> MGTVSSRRSWWPLPLLLLLLLLLGPAGARAQEDEDGDYEELVLALRSEEDGLAEAPEHGTTATFHRCAKDPWRLPGTYV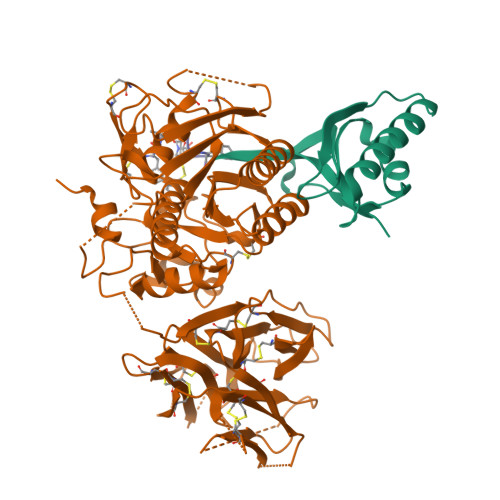VVLKEETHLSQSERTARRLQAQAARRGYLTKILHVFHGLLPGFLVKMSGDLLELALKLPHVDYIEEDSSVFAQ;> SIPWNLERITPPRYRADEYQPPDGGSLVEVYLLDTSIQSDHREIEGRVMVTDFENVPEEDGTRFHRQASKCDSHGTHLAGVVSGRDAGVAKGASMRSLRVLNCQGKGTVSGTLIGLEFIRKSQLVQPVGPLVVLLPLAGGYSRVLNAACQRLARAGVVLVTAAGNFRDDACLYSPASAPEVITVGATNAQDQPVTLGTLGTNFGRCVDLFAPGEDIIGASSDCSTCFVSQSGTSQAAAHVAGIAAMMLSAEPELTLAELRQRLIHFSAKDVINEAWFPEDQRVLTPNLVAALPPSTHGAGWQLFCRTVWSAHSGPTRMATAIARCAPDEELLSCSSFSRSGKRRGERMEAQGGKLVCRAHNAFGGEGVYAIARCCLLPQANCSVHTAPPAEASMGTRVHCHQQGHVLTGCSSHWEVEDLGTHKPPVLRPRGQPNQCVGHREASIHASCCHAPGLECKVKEHGIPAPQEQVTVACEEGWTLTGCSALPGTSHVLGAYAVDNTCVVRSRDVSTTGSTSEEAVTAVAICCRSRHLAQASQELQ> PPGTVAQSAPNLAGSRSYRETGTMTVTVDALNVRRAPNTSGEIVAVYKRGESFDYDTVIIDVNGYVWVSYIGGSGKRNYVATGATKDGKRFGNAWGTF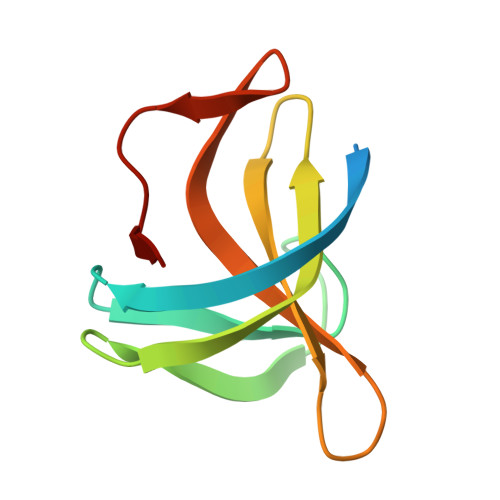K>[2x]MSYAEQSLPAANEAYVAAFGDKGSLPLPPGKRVAIVGCMDARLDTFGATGLHEGDA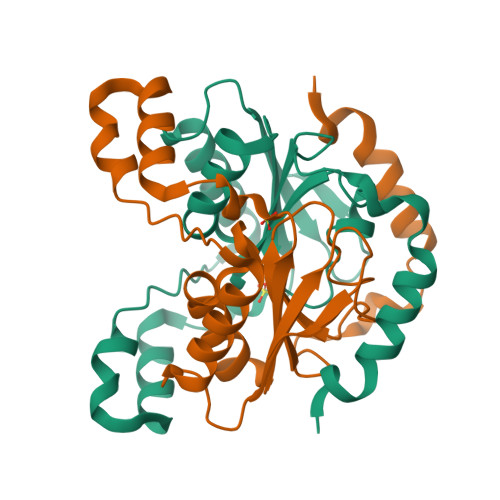HHIRNAGGRASDALRSLVISQELLGTREVIVIHHTDCGMLTFRSDQLHGLVKKRVAHEHFAAVDSLACLEFPDVDESIKEDVAFLKNHPLILPETVISGYRYEVETGKLVKIA> MELKNKKWTDEEFHKQREEVLQQWPTGKEVDLQEAVDYLKKIPAEKNFAEKLVLAKKKGITMAQPRAGVALLDEHIELLRYLQDEGGADFLPSTIDAYTRQNRYDECENGIKESEKAGRSLLNGFPGVNHGVKGCRKVLEAVNLPLQARHG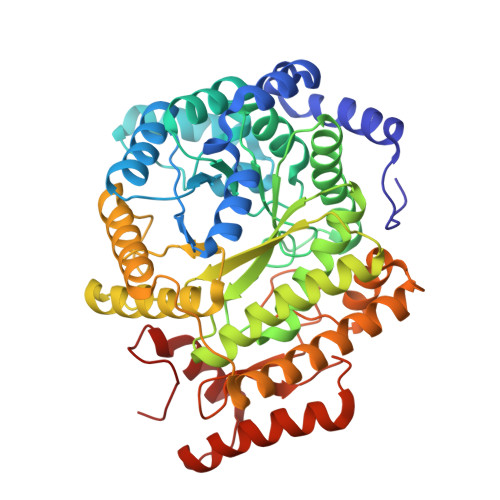TPDSRLLAEIIHAGGWTSNEGGGISYNVPYAKNVTIEKSLLDWQYCDRLVGFYEEQGVHINREPFGPLTGTLVPPSMSNAVGITEALLAAEQGVKNITVGYGECGNMIQDIAALRCLEEQTNEYLKAYGYNDVFVTTVFHQWMGGFPQDESKAFGVIVTATTIAALAGATKVIVKTPHEAIGIPTKEANAAGIKATKMALNMLEGQRMPMSKELETEMAVIKAETKCILDKMFELGKGDLAIGTVKAFETGVMDIPFGPSKYNAGKMMPVRDNLGCVRYLEFGNVPFTEEIKNYNRERLQERAKFEGRDVSFQMVIDDIFAVGKGRLIGRPE>[2x]MTLSPYLQEVAKRRTFAIISHPDAGKTTITEKVLLFGQAIQTAGTVKGRGSNQHAKSDWMEMEKQRGISITTSVMQFPYHDCLVNLLDTPGHEDFSEDTYRTLTAVDCCLMVIDAAKGVEDRTRKLMEVTRLRDTPILTFMNKLDRDIRDPMELLDEVENELKIGCAPITWPIGCGKLFKGVYHLYKDETYLYQSGKGHTIQEVRIVKGLNNPDLDAAVGEDLAQQLRDELE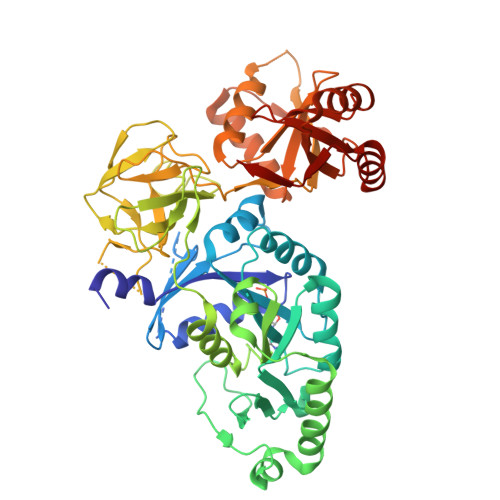LVKGASNEFDKELFLAGEITPVFFGTALGNFGVDHMLDGLVEWAPAPMPRQTDTRTVEASEDKFTGFVFKIQANMDPKHRDRVAFMRVVSGKYEKGMKLRQVRTAKDVVISDALTFMAGDRSHVEEAYPGDILGLHNHGTIQIGDTFTQGEMMKFTGIPNFAPELFRRIRLKDPLKQKQLLKGLVQLSEEGAVQVFRPISNNDLIVGAVGVLQFDVVVARLKSEYNVEAVYESVNVATARWVECADAKKFEEFKRKNESQLALDGGDNLAYIATSMVNLRLAQERYPDVQFHQTREH> MTTQLRYENNDDDERVEYNLFTNRSTMMANFEEWIKMATDNKINSRNSWNFALIDYFYDLDVLKDGENNINFQKASATLDGCIKIYSSRVDSVTTETGKLLSGLAQRKTNGASNGDDSNGGNGEGLGGDSDEANIEIDPLTGMPISNDPDVNNTRRRVYNRVLETTLVEFETIKMKELDQELIIDPLFKKALVDFDEGGAKSLLLNTLNIDNTARVIFDASIKDTQNVGQGKLQRKEEELIERDSLVDDENEPSQSLISTRNDSTVNDSVISAPSMEDEILSLGMDFIKFDQIAVCEISGSIEQLRNVVEDINQAKDFIENVNNRFDNFLTEEELQAAVPDNAEDDSDGFDMGMQQELCYPDENHDNTSHDEQDDDNVNSTTGSIFEKDLMAYF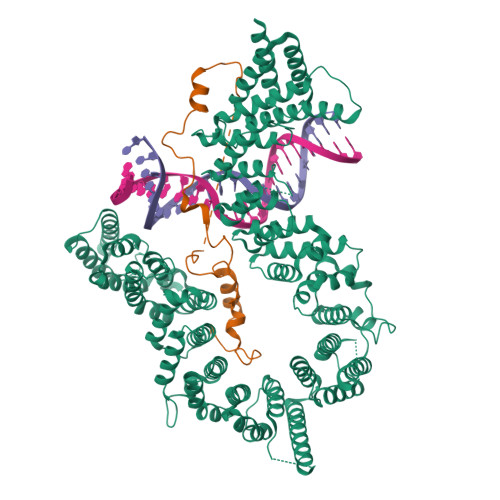DENLNRNWRGREHWKVRNFKKANLVNKESDLLEETRTTIGDTTDKNTTDDKSMDTKKKHKQKKVLEIDFFKTDDSFEDKVFASKGRTKIDMPIKNRKNDTHYLLPDDFHFSTDRITRLFIKPGQKMSLFSHRKHTRGDVSSGLFEKSTVSANHSNNDIPTIADEHFWADNYERKEQEEKEKEQSKEVGDVVGGALDNPFEDDMDGVDFNQAFEGTDDNEEASVKLDLQDDEDHKFPIRENKVTYSRVSKKVDVRRLKKNVWRSINNLIQEHDSRKNREQSSNDSETHTEDESTKELKFSDIIQGISKMYSDDTLKDISTSFCFICLLHLANEHGLQITHTENYNDLIVNYEDLATTQAAS;> MQDPDGIDINTKIFNSVAEVFQKAQGSYAGHRKHIAVLKKIQSKAVEQGYEDAFNFWFDKLVTKILPLKKNEIIGDRIVKLVAAFIASLERELILAKKQNYKLTNDEEGIFSRFVDQFIRHVLRGVESPDKNVRFRVLQLLAVIMDNIGEIDESLFNLLILSLNKRIYDREPTVRIQAVFCLTKFQDEEQTEHLTELSDNEENFEATRTLVASIQNDPSAEVRRAAMLNLINDNNTRPYILERARDVNIVNRRLVYSRILKSMGRKCFDDIEPHIFDQLIEWGLEDRELSVRNACKRLIAHDWLNALDGDLIELLEKLDVSRSSVCVKAIEALFQSRPDILSKIKFPESIWKDFTVEIAFLFRAIYLYCLDNNITEMLEENFPEASKLSEHLNHYILLRYHHNDISNDSQSHFDYNTLEFIIEQLSIAAERYDYSDEVGRRSMLTVVRNMLALTTLSEPLIKIGIRVMKSLSINEKDFVTMAIEIINDIRDDDIEKQEQEEKIKSKKINRRNETSVDEEDENGTHNDEVNEDEEDDNISSFHSAVENLVQGNGNVSESDIINNLPPEKEASSATIVLCLTRSSYMLELVNTPLTENILIASLMDTLITPAVRNTAPNIRELGVKNLGLCCLLDVKLAIDNMYILGMCVSKGNASLKYIALQVIVDIFSVHGNTVVDGEGKVDSISLHKIFYKVLKNNGLPECQVIAAEGLCKLFLADVFTDDDLFETLVLSYFSPINSSNEALVQAFAFCIPVYCFSHPAHQQRMSRTAADILLRLCVLWDDLQSSVIPEVDREAMLKPNIIFQQLLFWTDPRNLVNQTGSTKKDTVQLTFLIDVLKIYAQIEKKEIKKMIITNINAIFLSSEQDYSTLKELLEYSDDIAENDNLDNVSKNALDKLRNNLNSLIEEINERSETQTKDENNTANDQYSSILGNSFNKSSNDTIEHAADITDGNNTELTKTTVNISAVDNTTEQSNSRKRTRSEAEQIDTSKNLENMSIQDTSTVAKNVSFVLPDEKSDAMSIDEEDKDSESFSEVC> MAVKEDKQTDGDRWRGLAYDTSDDQQDITRGKGMVDSVFQAPMGTGTHHAVLSSYEYVSQGLRQYNLDNMMDGFYIAPAFMDKLVVHITKNFLTLPNIKVPLILGIWGGK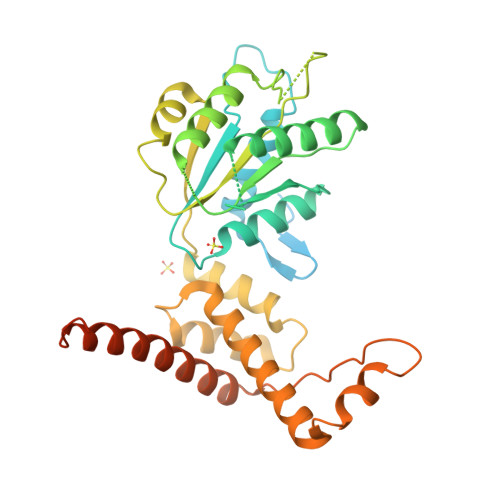GQGKSFQCELVMAKMGINPIMMSAGELESGNAGEPAKLIRQRYREAADLIKKGKMCCLFINDLDAGAGRMGGTTQYTVNNQMVNATLMNIADNPTNVQLPGMYNKEENARVPIICTGNDFSTLYAPLIRDGRMEKFYWAPTREDRIGVCKGIFRTDKIKDEDIVTLVDQFPGQSIDFFGALRARVYDDEVRKFVESLGVEKIGKRLVNSREGPPVFEQPEMTYEKLMEYGNMLVMEQENVKRVQLAETYLSQAALGDANADAIGRGTFYGGSAWSHPQFEK> MKHHHHHHHHHHGTSAGLEVLFQGPGNAIKLIHFLFRHKIIKFKTEIINFHEAYQQFVTIYEQYDDMVQEYLEIRTLLQLIQIKITNAQQRILDIEQKLSLATDHQKEFSQSLLQLKKPIEANLQMAE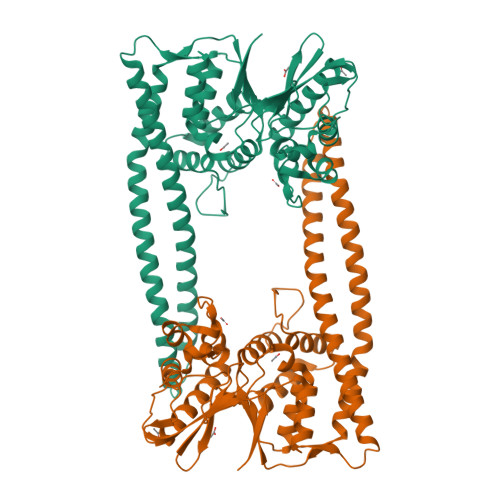KSKAGLEEKLSGLKTRLPSCIERFNKFMTQIEINDIKTLIRLLGDEVADRGSCDYFTLRILDFLYQNQIAIKIILSNHGYEFIHAYEKLVVGQPFKPKGYIGDIQIKSFWGLQLLLEQSVITEEELRSLVERAYKPTLKIIDYSLSEDGITLYSHAPIRFDSIRMAASQLGVTYNDSTKEALAETIDQLNAQLQIYMKNNMLHLLFENNEINDPTNMTDEERNASPLIYLVWNRWNESKEVENARPGKYNGYFVTYVHGHDPFQSPLTYVYNLDTL[(2~{R},3~{S},4~{R},5~{S})-3,4-bis(oxidanyl)-5-[4-[[[4-(phenylsulfonyl)phenyl]carbamoylamino]methyl]phenyl]oxolan-2-yl]methyl dihydrogen phosphate | 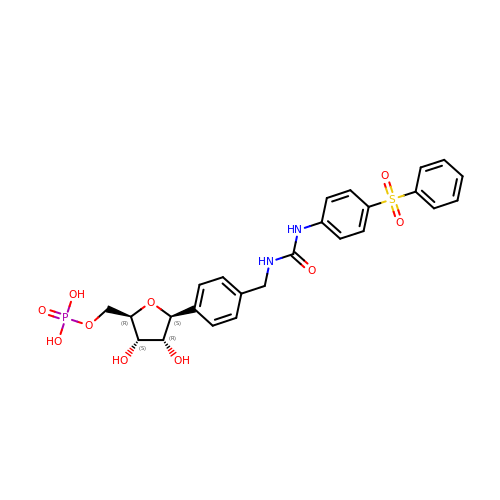C25 H27 N2 O10 P S | KYXDHJBRPDKXBZ-YCAMKHIRSA-N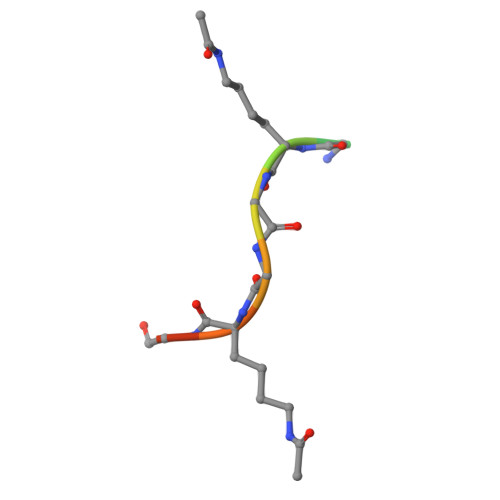> SGRGKGGKGLG> VGTQTGNPATNLPEAQGSASKEAEQSQNQAGETNGSIPVEVPKTDLDQAAKDAKSAGVNVVQDADVNKGTVKTAEEAVQKETEIKEDYTKQAEDIKKTTDQYKSDVAAHEAEVAKIKAKNQ;> QDLPTPPSVPTVHFHYFKLAVQPQVNKEIRNNNDINIDRTLVAKQSVVKFQLKTADLPAGRDETTSFVLVDPLPSGYQFNPEATKAASPGFDVTYDNATNTVTFKATAATLATFNADLTKSVATIYPTVVGQVLNDGATYKNNFTLTVNDAYGIKSNVVRVTTPGKPNDPDNPNNNYIKPTKVNKNENGVVIDGKTVLAGSTNYYELTWDLDQYKNDRSSADTIQKGFYYVDDYPEEALELRQDLVKITDANGNEVTGVSVDNYTNLEAAPQEIRDVLSKAGIRPKGAFQIFRADNPREFYDTYVKTG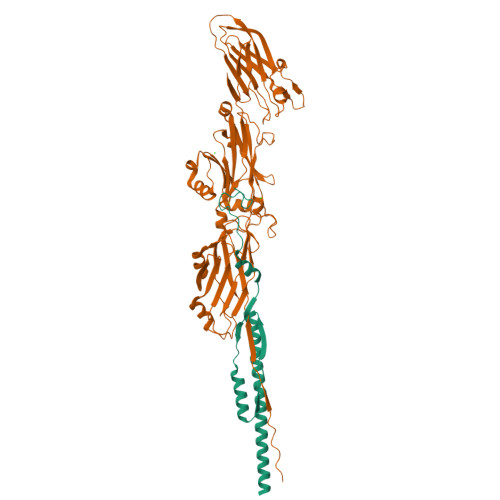IDLKIVSPMVVKKQMGQTGGSYENQAYQIDFGNGYASNIVINNVPKINPKKDVTLTLDPADTNNVDGQTIPLNTVFNYRLIGGIIPANHSEELFKYNFYDDYDQTGDHYTGQYKVFAKVDITLKNGVIIKSGTELTQYTTAEVDTTKGAITIKFKEAFLRSVSIDSAFQAESYIQMKRIAVGTFENTYINTVNGVTYSS>MAFTGKF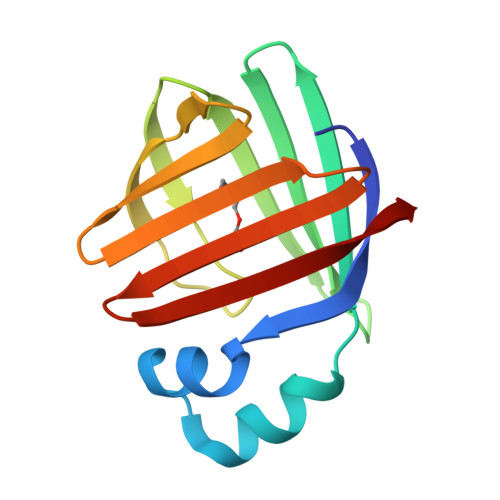EMESEKNYDEFMKLLGISSDVIEKARNFKIVTEVQQDGQDFTWSQHYSGGHTMTNKFTVGKESNIQTMGGKTFKATVQMEGGKLVVNFPNYHQTSEIVGDKLVEVSTIGGVTYERVSKRLA[3x]> SMKLDIKKTFSNRSDRVKGIDFHPTEPWVLTTLYSGRVEIWNYETQVEVRSIQVTETPVRAGKFIARKNWIIVGSDDFRIRVFNYNTGEKVVDFEAHPDYIRSIAVHPTKPYVLSGSDDLTVKLWNWENNWALEQTFEGHEHFVMCVAFNPKDPSTFASGCLDRTVKVWSLGQSTPNFTLTTGQERGVNYVDYYPLPDKPYMITASDDLTIKIWDYQTKSCVATLEGHMS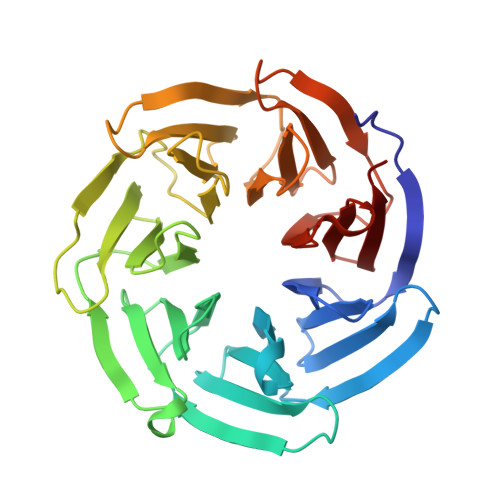NVSFAVFHPTLPIIISGSEDGTLKIWNSSTYKVEKTLNVGLERSWCIATHPTGRKNYIASGFDNGFTVLSLG> MASRADKASSIELKFDRNKGEVGDILIGTVRINNI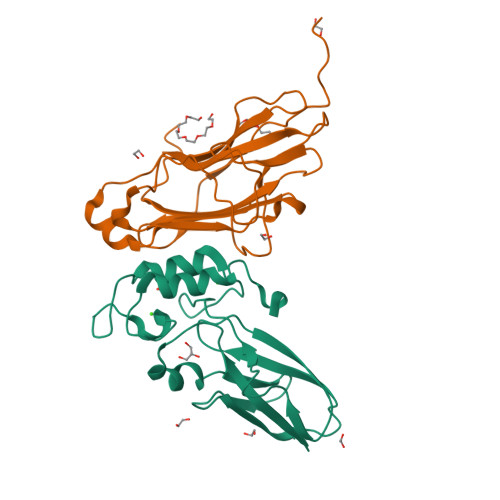KNFAGFQVNIVYDPKVLMAVDPETGKEFTSSTFPPGRTVLKNNAYGPIQIADNDPEKGILNFALAYSYIAGYKETGVTEESGIIAKIGFKILQKKSTAVKFQDTLSMPGAILGTQLFDWDGEVITGYEVIQPDVLSLGDEPYEVEHHHHHH;> MNNDSTDKTTVSGYISVDFDYPPESESKIKSGFNVKVAGTELSTKTDEKGYFEISGIPGDMREFTLEISKRNYLKRNVTVNGTGKLVVSTEDNPLILWAGDVERKGVQDNAINMVDVMEISKVFGTRAGDEEYVAELDLNMDGAINLFDIAIVIRHFNALPSRY>[2x]QRNSITAQRAPKSVKVIAVTPEEREAVMSIDFGGAYDFTSPGFNLFEVREKYSEPMDAAAGVVYNLLWNSGLPEKFGCREQTLLNFILQCRRRY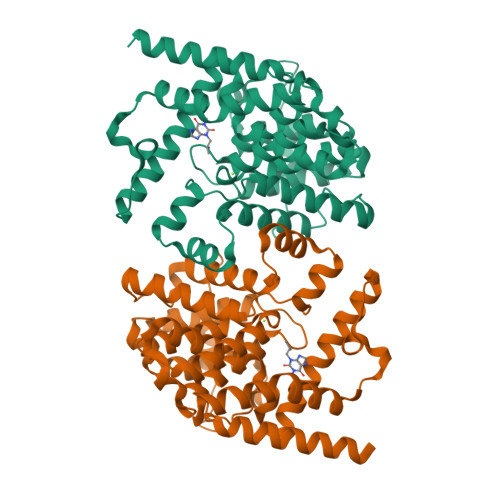RRVPYHNFYHVVDVCQTLHTYLYTGKASELLTELECYVLLVTALVHDLDHMGVNNSFYLKTDSPLGILSSASGNNSVLEVHHCSLAIEILSDPAADVFEGLSGQDVAYAYRALIDCVLATDMAKHADALSRFTELATSGFEKDNDTHRRLVMETLIKAGDVSNVTKPFETSRMWAMAVTEEFYRQGDMEKEKGVEVLPMFDRSKNNELARGQIGFIDFVAGKFFRDIVGNLFHGMQWCVDTVNSNRAKWQEILDGRRDSIRSSIV>MYSVKKSKSGYIFDKPRERIAFMFLKDGTYFMYHDGRILCYSLKPVDVSREELEEFERTGEPP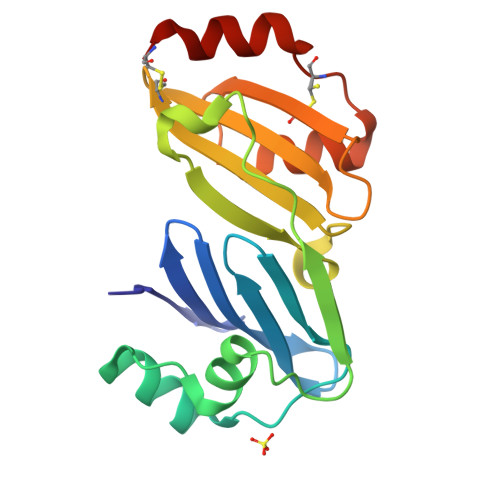ELIKRVKAGKYPENCVVKELPPIDKGLAQLNPNRKCVIIFTGFQDTVIDYVECNGETLAVARLIDEPGKVCRFAGKGNYKVAAVKLKRNEPCLTREEFLKKVEECRK[4x]> GSKDPGMLSRYEKWEKIKQHYQHWSDSLSEEGRGLLKKLQIPIEPKKDDIIHSLSQEEKELLKRIQIDSSDFLSTEEKEFLKKLQIDIRDSLSEEEKELLNRIQVDSSNPLSEKEKEFLKKLKLDIQPYDINQRLQDTGGLIDSPSINLDVRKQYKRDIQNIDALLHQSIGSTLYNKIYLYENMNINNLTATLGADLVDSTDNTKINRGIFNEFKKNFKYSISSNYMIVDINERPALDNERLKWRIQLSPDTRAGYLENGKLILQRNIGLEIKDVQIIKQSEKEYIRIDAKVVPKSKIDTKIQEAQLNINQEWNKALGLPKYTKLITFNVHNRYASNIVESAYLILNEWKNNIQSDLIKKVTNYLVDGNGRFVFTDITLPNIAEQYTHQDEIYEQVHSKGLYVPESRSILLHGPSKGVELRNDSEGFIHEFGHA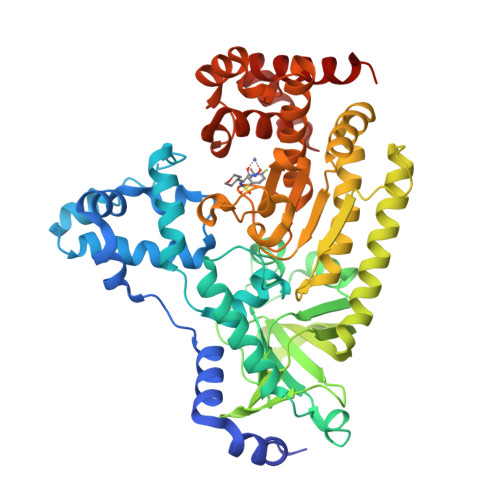VDDYAGYLLDKNQSDLVTNSKKFIDIFKEEGSNLTSYGRTNEAEFFAEAFRLMHSTDHAERLKVQKNAPKTFQFINDQIKFIINSLVPR>MEGWQRAFVLHSRPWSETSLMLDVFTEESGRVRLVAKGARSKRSTLKGALQPFTPLLLRFGGRGEVKTLRSAEAVSLALPLSGITLYSGLYINELLS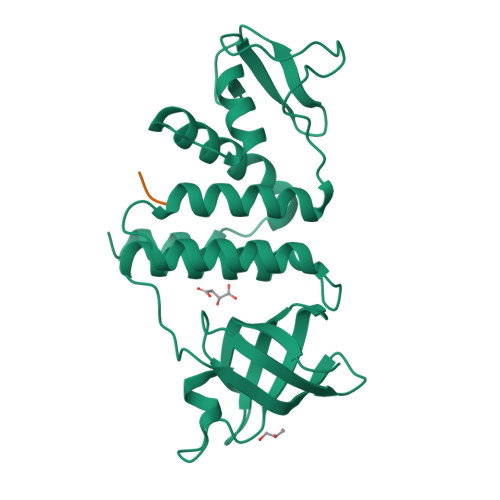RVLEYETRFSELFFDYLHCIQSLAGVTGTPEPALRRFELALLGHLGYGVNFTHCAGSGEPVDDTMTYRYREEKGFIASVVIDNKTFTGRQLKALNAREFPDADTLRAAKRFTRMALKPYLGGKPLKSRELFRQFMPKRTVKTHYE[2x];>[2x]YMDFDDDIPF> MR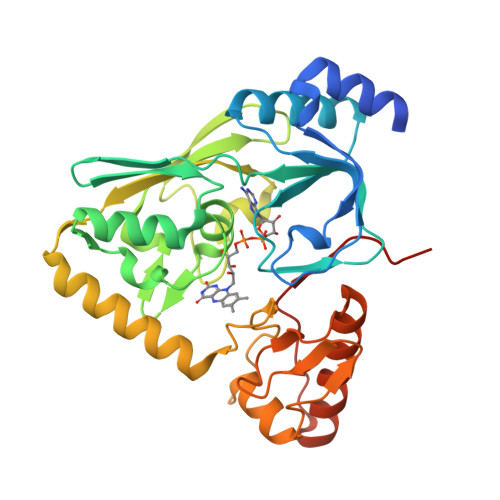GSHHHHHHTDPINKDIYQALQQLIPNEKIKVDEPLKRYTYTKTGGNADFYITPTKNEEVQAVVKYAYQNEIPVTYLGNGSNIIIREGGIRGIVISLLSLDHIEVSDDAIIAGSGAAIIDVSRVARDYALTGLEFACGIPGSIGGAVYMNAGAYGGEVKDCIDYALCVNEQGSLIKLTTKELELDYRNSIIQKEHLVVLEAAFTLAPGKMTEIQAKMDDLTERRESKQPLEYPSCGSVFQRPPGHFAGKLIQDSNLQGHRIGGVEVSTKHAGFMVNVDNGTATDYENLIHYVQKTVKEKFGIELNREVRIIGEHPKESLQPSLIS> SMCGSGGSTGGNTGGSTGGSTGGSTGNTQQLAVGIVLPTKDEPRWIQDETRFREALQQAGYQVEILFSQGSSAKEKENVEALIAKGIKVLIICPHDGTAAAAAAEAARAAGVKVISYDRLIRETDAVDYYVTFDSIAVGAQQAQYLVDHASGTGNPLYLYAGAASDNNAFLFFEGAWKVLQPKIADGTFVIKNSSEAVALQNKLDLTRDEMAKIIGQVTTNWDFNTAKNLAEANLTAATAADKGKVYILAPNDGTARAIADAFAADKDVT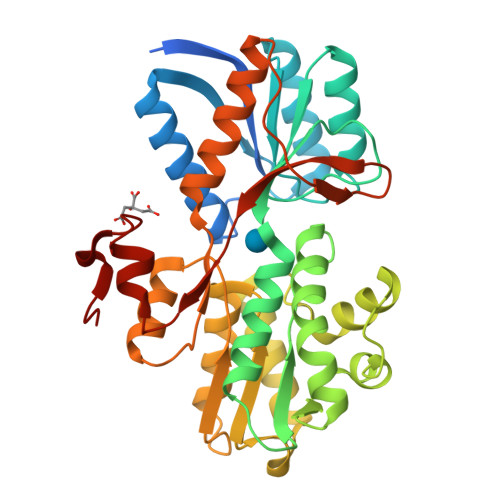EYFVTGQDAEKASVQYIIDGRQSMTVFKDVRTLVQDAIKAAVALLQDQQPEARGTYNNGKKDVPAIQSPVVTVTRDNVRAALIDSGYYSASDFTNLP>GAMGFNKILVVCVGN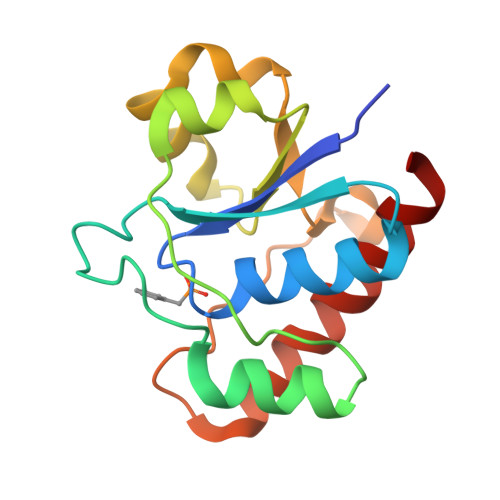ICRSPTGERVLQKLLPNKTVASAGIAAEKSRLIGKPADAMAIEVAKENCVDVENHQSQQLTSALCSQYDLILVMEKGHMEALTQIAPEARGKTMLFGQWIGQKDIPDPYRQSKEAFVHAYQLIDEAAQAWAKKL[4x]>[5x]MLVSVYLALLVACVGQAHSQANLMRLKSDLFNRSPMYPGPTKDDPLTVTLGFFLQDIVK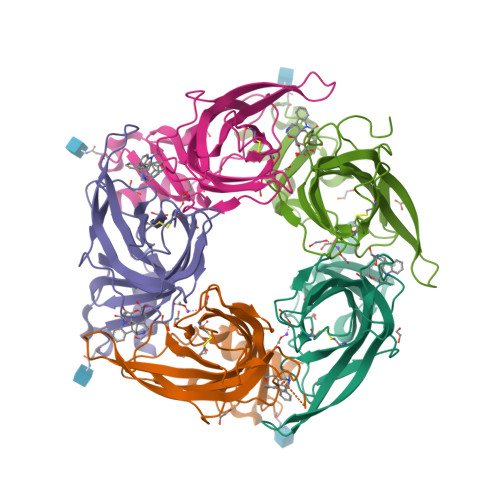VDSSTNEVDLVYYERQRWKLNSLMWDPNEYGNITDFRTSAADIWTPDITAASSTRPVQVLSPQIAVVTHDGSVMFSPAQRLSFMCDPTGVDSEEGVTCAVKFESWVYSGFEIDLKTDTDQVDLSSYYASSKYEILSATQTRQVQHYKGTGEPYIDVNLVVKFRERRAGNGFFRNLFDENLYFQGHHHHHH>GSISFHLPVNSRKCLREEIHKDLLVTGAYEITDQSGGAGGLRTHLKITDSAGHILYAKEDATKGK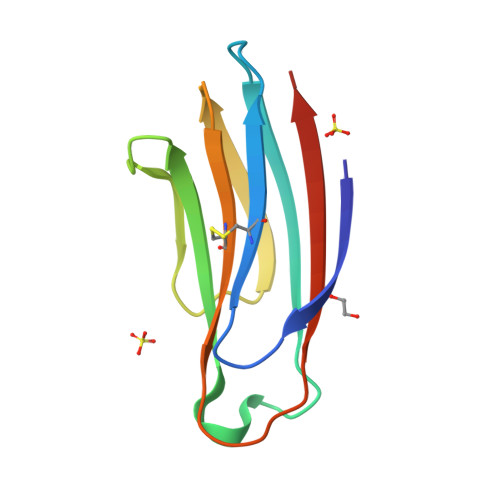FAFTTEDYDMFEVCFESKGTGRIPDQLVILDMKHGVEA[2x]> GTSTQTKAGSLTIVGTGIESIGQMTLQALSYIEAAAKVFYCVIDPATEAFILTKNKNCVDLYQYYDNGKSRLNTYTQMSELMVREVRKGLDVVGVFYGHPGVFVNPSHRALAIAKSEGYRARMLPGVSAEDCLFADLCIDPSNPGCLTYEASDFLIRDRPVSIHSHLVLFQVGCVGIADFNFTGFDNNKFGVLVDRLEQEYGAEHPVVHYIAAMMPHQDPVTDKYTVAQLREPEIAKRVGGVSTFYIPPKARKASNLDIIRRLELLPAGQVPDKKARIYPANQWEPDVPEVEPYRPSDQAAIAQLADHAPPEQYQPLATSKAMSDVMTKLALDPKALADYKADHRAFAQSVPDLTPQERAALELGDSWAIRCAMKNMPSSLLDAARESGEEASQNGFPAVIVVGVIGVIG

While chemical methylation of an amide bond uses a strong base to generate the imidate, OphA, the precursor protein of the fungal peptide macrocycle omphalotin A, self-hypermethylates amides at pH 7 using S-adenosyl methionine (SAM) as cofactor. Omphalotin A derives from the C terminus of the OphA protein, and it is the OphA protein that methylates its own C terminus using S-adenosyl methionine (SAM). The structure of OphA reveals a complex catenane-like arrangement in which the peptide substrate is clamped with its amide nitrogen aligned for nucleophilic attack on the methyl group of SAM. Here, we report the structure of the peptide amide methyltransferase OphA including complexes with cofactor [SAM and S-adenosyl homocysteine (SAH)], cofactor analog, substrate, and product.

Mutants Y63F, Y66F, Y76F, R72A, R72K, Y98A, Y98F, Q172A, and W400A of OphAΔC6 were expressed in E. coli. Superposition of both sinefungin complexes with the OphAΔC6 Y63F-SAH, OphAΔC18-SAM, and OphAΔC18-SAH complexes shows similar consistency in the protein structure, cofactor, and where present substrate positions. We conclude that the extensive hydrogen-bonding network at the active site and the catenane-like arrangement lead to a highly rigid active site. In both sinefungin complexes, the two nitrogen atoms (sinefungin and amide) approach close enough to form a hydrogen bond (distance varies between 3.1 and 3.3 Å).> GAASDEF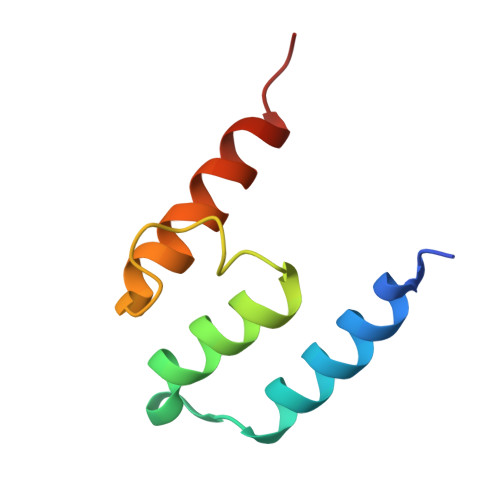ASEKVRLAQLTNKCNNNDLDYYIKESGDILGVTDKVKNKHDAKAILRYVLEELINFKKLNN>[2x]TDKR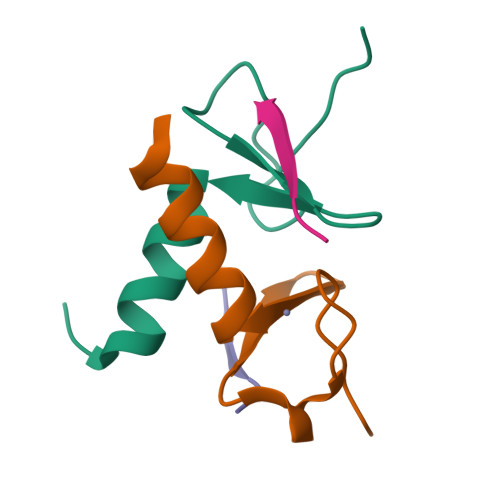KDGSGKLLYCSFCGKSQHEVRKLIAGPSVYICDECVDLCNDIIREEI;>APALRVVK[2x]>GDELYRQSLEIISRYLREQATGAKDTKPMGRSGATSRKALETLRRVGDGVQRNHETAFQGMLRKLDIKNEDDVKSLSRVMIHVFSDGVTNWGRIVTLISFGAFVAKHLKTINQESCIEPLAESITDVLVRTKRDWLVKQRGWD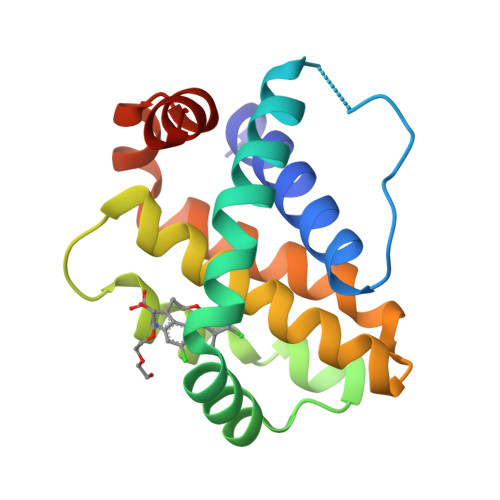GFVEFFHVED[6x]>[4x]MRIIMPVEFSRIVRDVERLIA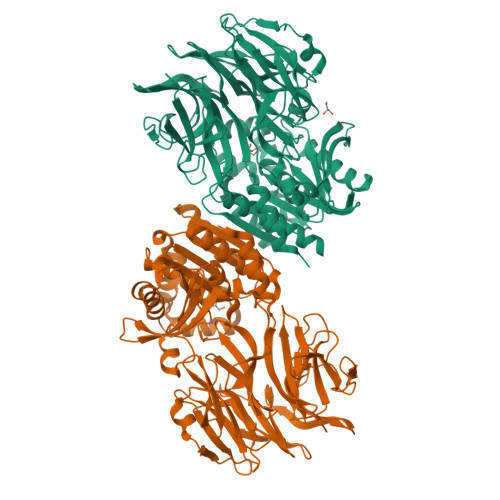VEKYSLQGVVDGDKLLVVGFSEGSVNAYLYDGGETVKLNREPINSVLDPHYGVGRVILVRDVSKGAEQHALFKVNTSRPGEEQRLEAVKPMRILSGVDTGEAVVFTGATEDRVALYALDGGGLRELARLPGFGFVSDIRGDLIAGLGFFGGGRVSLFTSNLSSGGLRVFDSGEGSFSSASISPGMKVTAGLETAREARLVTVDPRDGSVEDLELPSKDFSSYRPTAITWLGYLPDGRLAVVARREGRSAVFIDGERVEAPQGNHGRVVLWRGKLVTSHTSLSTPPRIVSLPSGEPLLEGGLPEDLRRSIAGSRLVWVESFDGSRVPTYVLESGRAPTPGPTVVLVHGGPFAEDSDSWDTFAASLAAAGFHVVMPNYRGSTGYGEEWRLKIIGDPCGGELEDVSAAARWARESGLASELYIMGYSYGGYMTLCALTMKPGLFKAGVAGASVVDWEEMYELSDAAFRNFIEQLTGGSREIMRSRSPINHVDRIKEPLALIHPQNASRTPLKPLLRLMGELLARGKTFEAHIIPDAGHAINTMEDAVKILLPAVFFLATQRERR> RYILPSFIEHSSFGVKESNPYNKLFEERIIFLGVQVDDASANDIMAQLLVLESLDPDRDITMYINSPGGGFTSLMAIYDTMQYVRADIQTVCLGQAASAAAVLLAAGTPGKRMALPNARVLIHQPSLSGVIQGQFSDLEI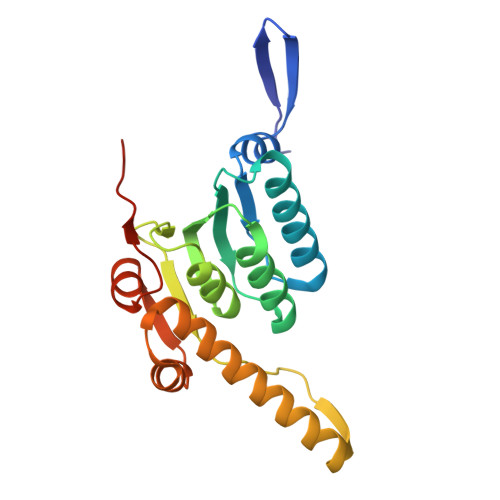QAAEIERMRTLMETTLARHTGKDAGVIRKDTDRDKILTAEEAKDYGIIDTVLEYRKLSAQTA> MIDLSKTVFYTSIDIGSRYIKGLVLGKRDQEWEALAFSSVKSRGLDEGEIKDAIAFKESVNTLLKELEEQLQKSLRSDFVISFSSVSFEREDTVIERDFGEEKRSITLDILSEMQSEALEKLKENGKTPLHIFSKRYLLDDERIVFNPLDMKASKIAIEYTSIVVPLKVYEMFYNF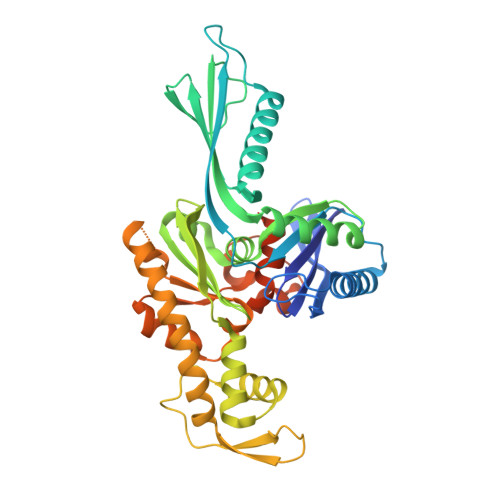LQDTVKSPFQLKSSLVSTAEGVLTTPEKDRGVVVVNLGYNFTGLIAYKNGVPIKISYVPVGMKHVIKDVSAVLDTSFEESERLIITHGNAVYNDLKEEEIQYRGLDGNTIKTTTAKKLSVIIHARLREIMSKSKKFFREVEAKIVEEGEIGIPGGVVLTGGGAKIPRINELATEVFKSPVRTGCYANSDRPSIINADEVANDPSFAAAFGNVFAVSENPYEETPVKSENPLKKIFRLFKELME>ATVQGGIEYRMPLPDGRVGLCSVGFPVTKGTIKGFATAGHCA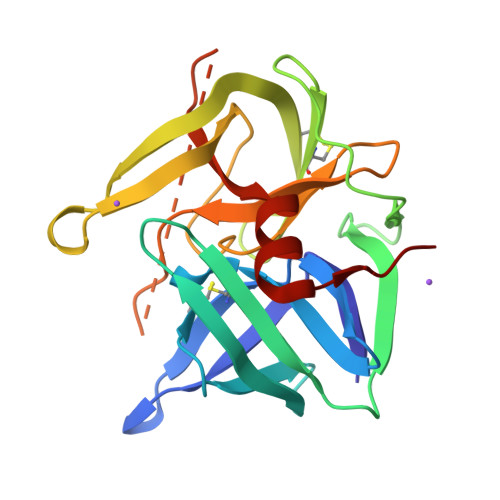KAGQSVQISGVNVGTFTASHFPNTDRAWVTIGAAHTLLGSVTNYTGGSVAVKGSTEAAIGAAVCRSGRTTQYKCGTITAKNVTVNYGTLGTVSGLTRANNCTGRGDSGGSWITAAGQAQGLTSGGNLPAGQNDNCSVPTSQRQTYFERINPVLSQYGLALVTS[2x]>GSSMGSQSLYREIHQLISFKDVLPDKNLLPDWSSNKNPCTFDGVTCRDDKVTSIDLSSKPLNVGFSAVSSSLLSLTGLESLFLSNSHINGSVSGFKCSASLTSLDLSRNSLSGPVTTLTSLGSCSGLKFLNVSSNTLDFPGKVSGGLKLNSLEVLDLSANSISGANVVGWVLSDGCGELKHLAISGNKISGDVDVSRCVNLEFLDVSSNNFSTGIPFLGDCSALQHLDISGNKLSGDFSRAISTCTELKLLNISSNQFVGPIPPLPLKSLQYLSLAENKFTGEIPDFLSGACDTLTGLDLSGNHFYGAVPPFFGSCSLLESLALSSNNFSGELPMDTLLKMRGLKVLDLSFNEFSGELPESLTNLSASLLTLDLSSNNFSGPILPNLCQNPKNTLQELYLQNNGFTGKIPPTLSNCSELVSLHLSFNYLSGTIPSSLGSLSKLRDLKLWLNMLEGEIPQELMYVKTLETLILDFNDLTGEIPSGLSNCTNLNWISLSNNRLTGEIPKWIGRLENLAILKLSNNSFSGNIPAELGDCRSLIWLDLNTNLFNGTIPAAMFKQSGKIAANFIAGKRYVYIKNDGMKKECHGAGNLLEFQGIRSEQLNRLSTRNPCNITSRVYEGHTSPTFDNNGSMMFLDMSYNMLSGYIPKEIGSMPYL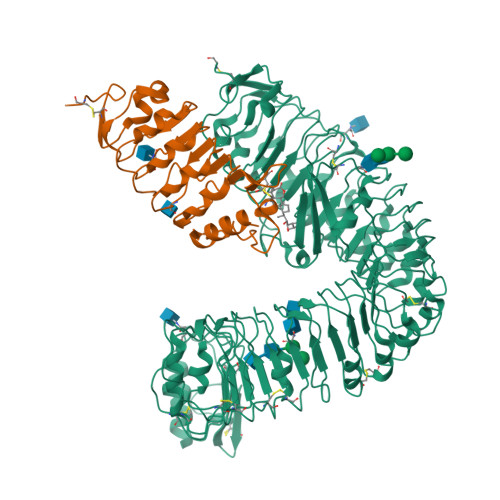FILNLGHNDISGSIPDEVGDLRGLNILDLSSNKLDGRIPQAMSALTMLTEIDLSNNNLSGPIPEMGQFETFPPAKFLNNPGLCGYPLPRCDPSNADGYAHHQRSHGRRLENLYFQGA[2x];>GSSMASANLEGDALHTLRVTLVDPNNVLQSWDPTLVNPCTWFHVTCNNENSVIRVDLGNAELSGHLVPELGVLKNLQYLELYSNNITGPIPSNLGNLTNLVSLDLYLNSFSGPIPESLGKLSKLRFLRLNNNSLTGSIPMSLTNITTLQVLDLSNNRLSGSVPDNGSFSLFTPISFANNLDLCGPVTSHPCPGSLENLYFQGA[2x]>[2x]KGTSENKSTTATDTVQAEKPQSGTIHLTRAEFLKKIADYENHSKEWKYLGDKPAIVDFYADWCGPCKMVAPILEELSKEYAGKIYIYKVNVDKEPELARDFGI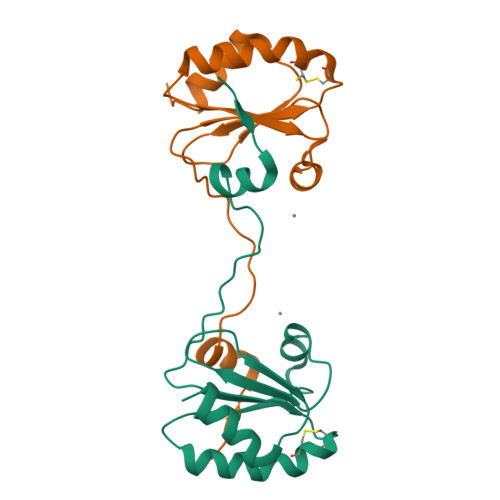QSIPTIWFVPMKGEPQVNMGALSKEQLKGYIDKVLLKQ>[4x]GPHMA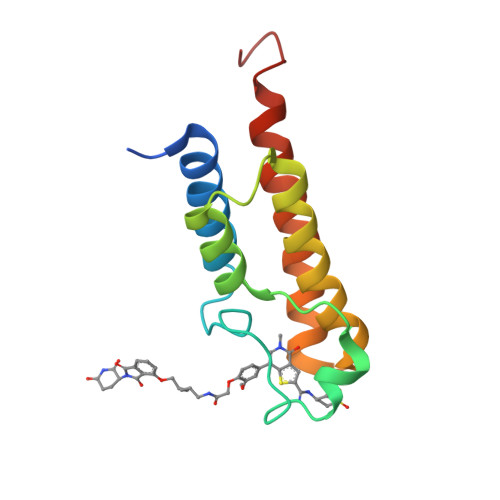ENESTPIQQLLEHFLRQLQRKDPHGFFAFPVTDAIAPGYSMIIKHPMDFGTMKDKIVANEYKSVTEFKADFKLMCDNAMTYNRPDTVYYKLAKKILHAGFKMMSKQAALLGNEDTA> MNDRDFMRYSRQILLDDIALDGQQKLLDSQVLIIGLGGLGTPAALYLAGAGVGTLVLADDDDVHLSNLQRQILFTTEDIDRPKSQVSQQRLTQLNPDIQLTALQQRLTGEALKDAVARADVVLDCTDNMATRQEINAACVALNTPLITASAVG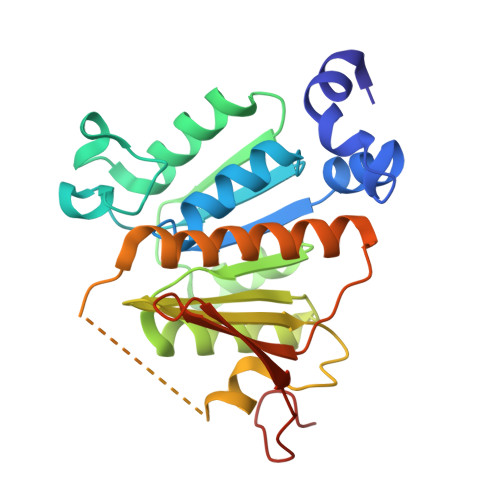FGGQLMVLTPPWEQGCYRCLWPDNQEPERNCRTAGVVGPVVGVMGTLQALEAIKLLSGIETPAGELRLFDGKSSQWRSLALRRASGCPVCGGSNADPV> MAHHHHHHMSDEDHDFAHQGGGDNAS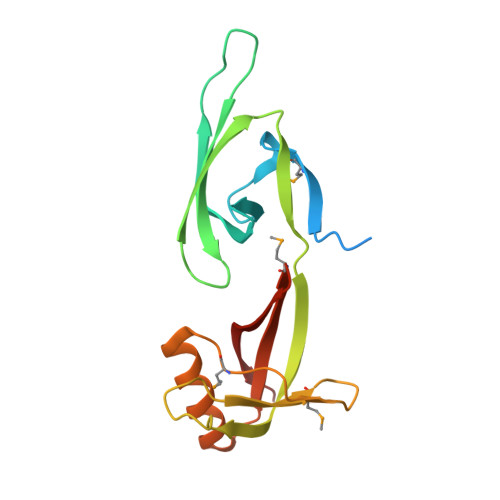KTYPMAAGALKKGGYVCINGRPCKVIDLSVSKTGKHGHAKVSIVATDIFTGNRLEDQAPSTHNVEVPFVKTFTYSVLDIQPNEDPSLPSHLSLMDDEGESREDLDMPPDAALATQIKEQFDSGKEVLVVVVSAMGTEQVLQTKNAAEK> CGCGACCUCAGAUCAGACGUGGCGACCCGCUGAAUUUAAGCAUAUUAGUCAGCGGAGGAGAAGAAACUAACCAGGAUUCCCUCAGUAACGGCGAGUGAACAGGGAAGAGCCCAGCGCCGAAUCCCCGCCCCGCGGCGGGGCGCGGGACAUGUGGCGUACGGAAGACCCGCUCCCCGGCGCCGCUCGUGGGGGGCCCAAGUCCUUCUGAUCGAGGCCCAGCCCGUGGACGGUGUGAGGCCGGUAGCGGCCCCCGGCGCGCCGGGCCCGGGUCUUCCCGGAGUCGGGUUGCUUGGGAAUGCAGCCCAAAGCGGGUGGUAAACUCCAUCUAAGGCUAAAUACCGGCACGAGACCGAUAGUCAACAAGUACCGUAAGGGAAAGUUGAAAAGAACUUUGAAGAGAGAGUUCAAGAGGGCGUGAAACCGUUAAGAGGUAAACGGGUGGGGUCCGCGCAGUCCGCCCGGAGGAUUCAACCCGGCGGCGGGUCCGGCCGUGUCGGCGGCCCGGCGGAUCUUUCCCGCGCGGGGGACCGUCCCCCGACCGGCGACCGGCCGCCGCCGGGCGCAUUUCCACCGCGGCGGUGCGCCGCGACCGGCUCCGGGACGGCUGGGGAAGGCCCGGCGGGGAAGGUGGCUCGGGGGCCCCCGAGUGUUACAGCCCCCCCGGCAGCAGCACUCGCCGAAUCCCGGGGCCGAGGGAGCGAGACCCGUCGCCGCGCUCUCCCCCCUCCCGGCGCGCCGGGGGGGGCCGGGCCACCCCUCCCACGGCGCGACCGCUCGGGGCGGACUGUCCCCAGUGCGCCCCGGGCGGGUCGCGCCGUCGGGCCCGGGGGAGGCCACGCGCGCGUCCCCCGAAGAGGGGGACGGCGGAGCGAGCGCACGGGGUCGGCGGCGACGUCGGCUACCCACCCGACCCGUCUUGAAACACGGACCAAGGAGUCUAACACGUGCGCGAGUCGGGGGCUCGCACGAAAGCCGCCGUGGCGCAAUGAAGGUGAAGGCCGGCGCGCUCGCCGGCCGAGGUGGGAUCCCGAGGCCUCUCCAGUCCGCCGAGGGCGCACCACCGGCCCGUCUCGCCCGCCGCGCCGGGGAGGUGGAGCACGAGCGCACGUGUUAGGACCCGAAAGAUGGUGAACUAUGCCUGGGCAGGGCGAAGCCAGAGGAAACUCUGGUGGAGGUCCGUAGCGGUCCUGACGUGCAAAUCGGUCGUCCGACCUGGGUAUAGGGGCGAAAGACUAAUCGAACCAUCUAGUAGCUGGUUCCCUCCGAAGUUUCCCUCAGGAUAGCUGGCGCUCUCGCAGACCCGACGCCCGCCACGCAGUUUUAUCCGGUAAAGCGAAUGAUUAGAGGUCUUGGGGCCGAAACGAUCUCAACCUAUUCUCAAACUUUAAAUGGGUAAGAAGCCCGGCUCGCUGGCGUGGAGCCGGGCGUGGAAUGCGAGUGCCUAGUGGGCCACUUUUGGUAAGCAGAACUGGCGCUGCGGGAUGAACCGAACGCCGGGUUAAGGCGCCCGAUGCCGACGCUCAUCAGACCCCAGAAAAGGUGUUGGUUGAUAUAGACAGCAGGACGGUGGCCAUGGAAGUCGGAAUCCGCUAAGGAGUGUGUAACAACUC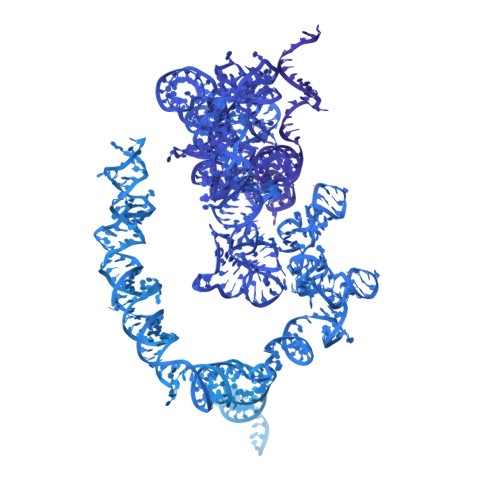ACCUGCCGAAUCAACUAGCCCUGAAAAUGGAUGGCGCUGGAGCGUCGGGCCCAUACCCGGCCGUCGCCGGCAGUCGAGAGUGGACGGGAGCGGCGGGCCGGAGCCCCGCGGACGCUACGCCGCGACGAGUAGGAGGGCCGCUGCGGUGAGCCUUGAAGCCUAGGGCGCGGGCCCGGGUGGAGCCGCCGCAGGUGCAGAUCUUGGUGGUAGUAGCAAAUAUUCAAACGAGAACUUUGAAGGCCGAAGUGGAGAAGGGUUCCAUGUGAACAGCAGUUGAACAUGGGUCAGUCGGUCCUGAGAGAUGGGCGAGCGCCGUUCCGAAGGGACGGGCGAUGGCCUCCGUUGCCCUCGGCCGAUCGAAAGGGAGUCGGGUUCAGAUCCCCGAAUCCGGAGUGGCGGAGAUGGGCGCCGCGAGGCGUCCAGUGCGGUAACGCGACCGAUCCCGGAGAAGCCGGCGGGAGCCCCGGGGAGAGUUCUCUUUUCUUUGUGAAGGGCAGGGCGCCCUGGAAUGGGUUCGCCCCGAGAGAGGGGCCCGUGCCUUGGAAAGCGUCGCGGUUCCGGCGGCGUCCGGUGAGCUCUCGCUGGCCCUUGAAAAUCCGGGGGAGAGGGUGUAAAUCUCGCGCCGGGCCGUACCCAUAUCCGCAGCAGGUCUCCAAGGUGAACAGCCUCUGGCAUGUUGGAACAAUGUAGGUAAGGGAAGUCGGCAAGCCGGAUCCGUAACUUCGGGAUAAGGAUUGGCUCUAAGGGCUGGGUCGGUCGCGGCCGGCGCCUAGCAGCCGACUUAGAACUGGUGCGGACCAGGGGAAUCCGACUGUUUAAUUAAAACAAAGCAUCGCGAAGGCCCGCGGCGGGUGUUGACGCGAUGUGAUUUCUGCCCAGUGCUCUGAAUGUCAAAGUGAAGAAAUUCAAUGAAGCGCGGGUAAACGGCGGGAGUAACUAUGACUCUCUUAAGGUAGCCAAAUGCCUCGUCAUCUAAUUAGUGACGCGCAUGAAUGGAUGAACGAGAUUCCCACUGUCCCUACCUACUAUCCAGCGAAACCACAGCCAAGGGAACGGGCUUGGCGGAAUCAGCGGGGAAAGAAGACCCUGUUGAGCUUGACUCUAGUCUGGCACGGUGAAGAGACAUGAGAGGUGUAGAAUAAGUGGGAGGCCCCCGGCGCCCCCCCGGUGUCCCCGCGAGGGGCCCGGGGCGGGGUCCGCCGGCCCUGCGGGCCGCCGGUGAAAUACCACUACUCUGAUCGUUUUUUCACUGACCCGGUGAGGCGGGGGGGCGAGCCCCGAGGGGCUCUCGCUUCUGGCGCCAAGCGCCCGGCCGCGCGCCGGCCGGGCGCGACCCGCUCCGGGGACAGUGCCAGGUGGGGAGUUUGACUGGGGCGGUACACCUGUCAAACGGUAACGCAGGUGUCCUAAGGCGAGCUCAGGGAGGACAGAAACCUCCCGUGGAGCAGAAGGGCAAAAGCUCGCUUGAUCUUGAUUUUCAGUACGAAUACAGACCGUGAAAGCGGGGCCUCACGAUCCUUCUGACCUUUUGGGUUUUAAGCAGGAGGUGUCAGAAAAGUUACCACAGGGAUAACUGGCUUGUGGCGGCCAAGCGUUCAUAGCGACGUCGCUUUUUGAUCCUUCGAUGUCGGCUCUUCCUAUCAUUGUGAAGCAGAAUUCACCAAGCGUUGGAUUGUUCACCCACUAAUAGGGAACGUGAGCUGGGUUUAGACCGUCGUGAGACAGGUUAGUUUUACCCUACUGAUGAUGUGUUGUUGCCAUGGUAAUCCUGCUCAGUACGAGAGGAACCGCAGGUUCAGACAUUUGGUGUAUGUGCUUGGCUGAGGAGCCAAUGGGGCGAAGCUACCAUCUGUGGGAUUAUGACUGAACGCCUCUAAGUCAGAAUCCCGCCCAGGCGGAACGAUACGGCAGCGCCGCGGAGCCUCGGUUGGCCUCGGAUAGCCGGUCCCCCGCCGGGGUCCGGUGCGGAGUGCCCUUCGUCCUGGGAAACGGGGCGCGGCCGGAGAGGCGGCCGCCCCCUCGCCCGUCACGCACCGCACGUUCGUGGGGAACCUGGCGCUAAACCAUUCGUAGACGACCUGCUUCUGGGUCGGGGUUUCGUACGUAGCAGAGCAGCUCCCUCGCUGCGAUCUAUUGAAAGUCAGCCCUCGACACAAGGGUUUGU>SNAMDQQFVAQLEQALGAIVQPTGSLKDATKTLQSQFYTQSAALPALIHILQNSSNDGIKQLAGVEARKQVSKHWGSLDAATQTSVKQSLLNSAFNEGKDAVRHANARVIASIGSEELDEKKWPELIPNLLQAACDSNPKIRETAIFIILSLLESFNANLALHIDDFLNLFAQTINDSASLETRSLSAQALSYVSSLIEEEGEINPQYAAKFASLIPSVVQVLDATIREGDTTNTKLIFNCLNDFLLLDSQLTGNTIADLVKLALQIAVNSDVDEDIRVFAVQFVTSALVYRKSKINQAKLGPEITLAALKVASEEIDVEDELTNEDEAGENEENTPALTALRLISNASGELSPSQVGVPIIEHLPTMLSSSNPFERRSILLAISVLVTGSPDYTLSQFDKIIPATVTGLKDSEAVVQLAALKCIVQLSTNLQDEVARYHEQYLPLVIDIIDSAKHVVIYKYATLALDGLLEFIAHNDIIKYLDPLMNKLFQMLETQQSPKLRAAIVSAIGSCAFAAGSGFVPYFKTSVQYLQQFIQNVSQIEGLSEDDIELKALTFENISTMGRAVKSAAFAEYAEPLVNAAYEAIKTDSARLRESGYAFIANMAKVYGKDFAPFLQTIIPEIFKTLEQEEYQFNFDGDEDFLEGIEDLDEEELQSKFTVNTGIAYEKEVAAAALSELAIASKEHFLEYVEPSLKVLAEQVNESYGLKETALHSMWAIVKAVLLTANLKEGEYPKGVPSGSYVDASALAVIQTVREVSLNNVIEEVETSMVISVFQDLSEMLRLFGPIIIMDNGDSTHLDQLCREALSVLKGEHACQTIHFEEDVPEDEDLDASETEATLLDVALDIYVALSTNLVGGFAQVFTTAKPVILQLCQSKSKNKRSFAVGALSEIALGMRDENPFIQELLEALIISLTNDKSLEVRCNASYGVGLLIEYSSFDVSAIYSPVLKSLYEILSVADEKNLATEDDEATKEIVDRTFSNVCGCVARMILKHQNLVPLEHTIPALLSHLPFNTAFEEYDPIFKLFLKLFQEQNSTIINEAPKVIAIFATVFEKESERIELETNSTLGREENLEKRKQFQSEEIKQQVIELLKHLNQQFNGAVAQNPVLAQVIA[2x]

Kap123, the most abundant karyopherin in budding yeast, functions as a primary transporter for the H3:H4/Asf1 complex, whereas Kap121 acts as a secondary transporter. Kap proteins share the common structural motif of helical tandem HEAT (Huntingtin, elongation factor 3 (EF3), protein phosphatase 2A (PP2A), and the yeast kinase TOR1) repeats with a right-handed superhelical solenoid structure. Here, we report crystal structures of full-length Kluyveromyces lactis (Kl) Kap123 alone and in complex with NLS peptides of H3 and H4. We identify that there are two spatially separated lysine-binding pockets within Kap123 that specifically interact with H3- and H4-NLSs.

The crystal structure of full length Kl Kap123 was determined using the single-wavelength anomalous diffraction (SAD) method and refined at 2.35 Å resolution with a crystallographic R value of 20.99% and a free R value of 23.49%. Crystals contain two copies of full-length Kl Kap123 per asymmetric unit. The refined structure displays 24 tandem HEAT repeats with a right-handed superhelical solenoid structure. The first HEAT repeat (residues 1–39), an intra-loop of repeat 8 (residues 325–329), repeat 15 (residues 631–656) and repeat 18 (residues 818–828) are disordered in the final structure. The overall architecture of Kl Kap123 is similar to other known karyopherin structures, excepting repeat 23. The unique extra-long helix of repeat 23 is conserved in budding yeasts, such as Saccharomyces cerevisiae and K. lactis, and establishes an intra-molecular interaction with repeats 12–14 using electrostatic and hydrogen bond interactions. This interaction may further stabilize the superhelical architecture of Kl Kap123. However, the dynamic behavior of Kap123 is thought to be restricted owing to intramolecular interactions between repeats 12 and 14 and the extended helix of the repeat 23. This extended helix restricts the distance in-between two lysine-binding pockets.>[2x]SNAESRFLDTWRWQNYFLLH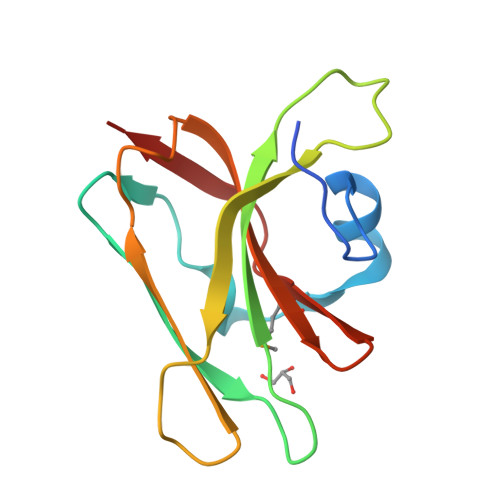HNADFIEELAVGDLKHGDTFDVTIYTGGKDTGIVKIYQLSGNENDEINLHRYKTIYDSGLKHNYGRFVTPITKAYNPGTYVAVMKLGENYYYGGSFKISK>MGSVEIPTKVLTNTSSQLKMPVVGMGSAPDFTCKKDTKDAIIEAIKQGYRHFDTAAAYGSEQALGEALKEAIELGLVTRDDLFVTSKLWVTENHPHLVIPALQKSLKTLQLDYLDLYLIHWPLSSQPGKFSFPIDVADLLPFDVKGVWESMEESLKLGLTKAIGVSNFSVKKLENLLSVATVLPAVNQVEMNLAWQQKKLREFCNAHGIVLTAFSPVRKGASRGPNEVMENDMLKEIADAHGKSVAQISLRWLYEQGVTFVPKSYDKERMNQNLRIFDWSLTKEDHEKIAQIKQNRLIPGP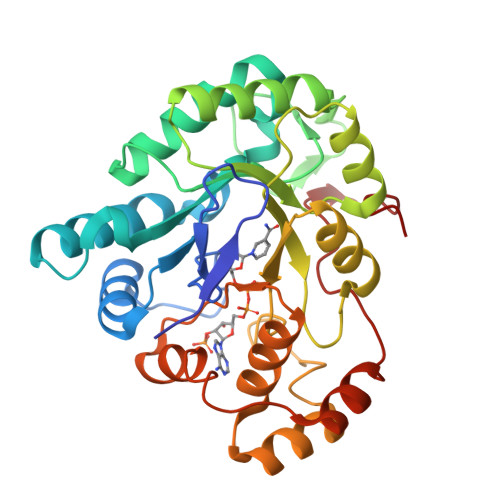TKPGLNDLYDD[2x]> GHMDQSDFSPYIEIDLPSESRIQSLHKSGLAAQEWVACEKVHGTNFGIYLINQGDHEVVRFAKRSGIMDPNENFFGYHILIDEFTAQIRILNDLLKQKYGLSRVGRLVLNGELFGAKYKHPLVPKSEKWCTLPNGKKFPIAGVQIQREPFPQYSPELHFFAFDIKYSVSGAEEDFVLLGYDEFVEFSSKVPNLLYARALVRGTLDECLA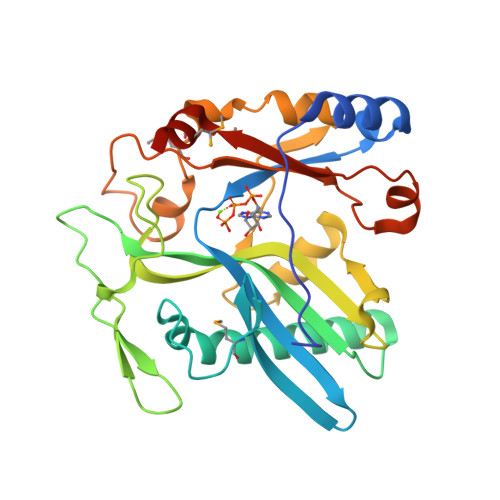FDVENFMTPLPALLGLGNYPLEGNLAEGVVIRHVRRGDPAVEKHNVSTIIKLRCSSFMELKHPGKQKE> MVEFKILEKRPDSIKFIVSGVDVPFANALRRTILSEVPTFAVDEVEFLENDSALFDEIIAHRLAMIPLTTPHERFSLDALELDDYTVTLSLEAEGPGMVYSGDLKSSDGDVKPANPNIPIVKLAEGQRLTFNAYARLGRGKDH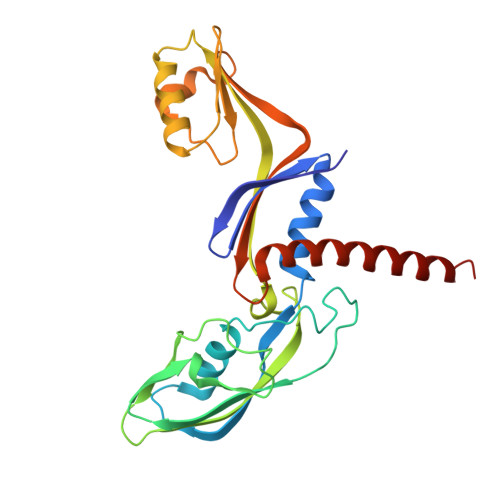AKWQPGFVYYKYLTKIHVSKDVPDWEELKELAERRGLPVEESDEEIVITTIKAFYLPRKFEEHMGKGIREEIVPGSFVFTVETNGELPVEEIVSIALKILMRKSDRFINELHKLAD> MKKEKIDLFYGALLHNIGKVIQRATGERKKHALVGADWFDEIADNQVISDQIRYHMANYQSDKLGNDHLAYITYIADNIASGVDRRQSNEESDEDTSAKIWDTYTNQADIFNVFGAQTDKRYFKPTVLNLKSKPNFASATYEPFSKGDYAAIATRIKNELAEFEFNQVQIDSLLNLFEATLSFVPSSTNTKEIADISLADHSRLTAAFALAIYDYLEDKGRHNYKEDLFTKVSAFYEEEAFLLASFDLSGIQDFIYNINIATNGAAKQLKARSLYLDFMSEYIADSLLDKLGLNRANMLYVGGGHAYFVLANTEKTVETLVQFEKDFNQFLLANFQTRLYVAFGWGSFAAKDIMSELNSPESYRQVYQKASRMISKKKISRYDYQTLMLLNRGGKSSERECEICHSVENLVSYHDQKVCDICRGLYQFSKEIAHDHFIITENEGLPIGPNACLKGVAFEKLSQEAFSRVYVKNDYKAGTVKATHVFVGDYQCDEIYNYAALSKNENGLGIKRLAVVRLDVDDLGAAFMAGFSQQGNGQYSTLSRSATFSRSMSLFFKVYINQFASDKKLSIIYAGGDDVFAIGSWQDIIAFTVELRENFIKWTNGKLTLSAGIGLFADKTPISLMAHQTGELEEAAKGNEKDSISLFSSDYTFKFDRFITNVYDDKLEQIRYFFNHQDERGKNFIYKLIELLRNHDRMNMARLAYYLTRLEELTRETDRDKFKTFKNLFYSWYTNKNDKDRKEAELALLLYIYEIRKD;> MTYKLYIMTFQNAHFGSGTLDSSKLTFSADRIFSALVLEALKMGKLDAFLAEANQDKFTLTDAFPFQFGPFLPKPIGY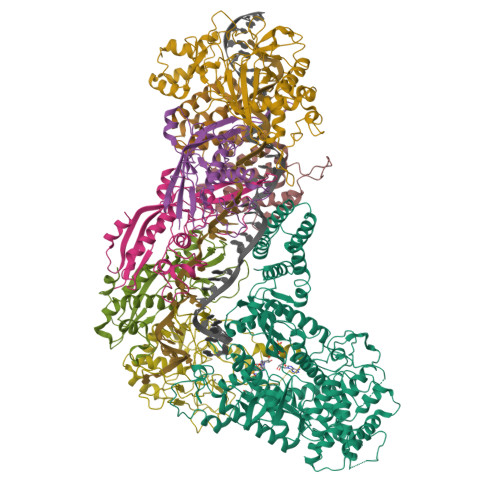PKHDQIDQSVDVKEVRRQAKLSKKLQFLALENVDDYLNGELFENEEHAVIDTVTKNQPHKDDNLYQVATTRFSNDTSLYVIANESDLLNELMSSLQYSGLGGKRSSGFGRFELDIQNIPLELSDRLTKNHSDKVMSLTTALPVDADLEEAMEDGHYLLTKSSGFAFSHATNENYRKQDLYKFASGSTFSKTFEGQIVDVRPLDFPHAVLNYAKPLFFKLEV;>[2x]MTILTDENYVDIAEKAILKLERNTRNRKNPDAFFLTTSKLRNLLSLTSTLFDESKVKEYDALLDRIAYLRVQFVYQAGREIAVKDLIEKAQILEALKEIKDRETLQRFCRYMEALVAYFKFYGGKD;>[3x]MTFAKIKFSAQIRLETGLHIGGSDAFAAIGAINSPVIKDPITNLPIIPGSSLKGKMRTLLAKVYNEKVAEKPSDDSDILSRLFGNSKDKRFKMGRLIFRDAFLSNADELDSLGVRSYTEVKFENTIDRITAEANPRQIERAIRNSTFDFELIYEITDENENQVEEDFKVIRDGLKLLELDYLGGSGSRGYGKVAFENLKATTVFGNYDVKTLNELLTAEV;> MKNDYRTFKLSLLTLAPIHIGNGEKYTSREFIYENKKFYFPDMGKFYNKMVEKRLAEKFEAFLIQTRPNARNNRLISFLNDNRIAERSFGGYSISETGLESDKNPNSAGAINEVNKFIRDAFGNPYIPGSSLKGAIRTILMNTTPKWNNENAVNDFGRFPKENKNLIPWGPKKGKEYDDLFNAIRVSDSKPFDNKSLILVQKWDYSAKTNKAKPLPLYRESISPLTKIEFEITTTTDEAGRLIEELGKRAQAFYKDYKAFFLSEFPDDKIQANLQYPIYLGAGSGAWTKTLFKQADGILQRRYSRMKTKMVKKGVLKLTKAPLKTVKIPSGNHSLVKNHESFYEMGKANFMIKEIDK>MTVQCKPIPALYTVYVLRSTVRHASLYIGSTPNPPRRLKQHNGLVPGGAARTSRSSLRPWEMVALVSGFPSMVAALKFQWALTNPHLSVHIPSASRLTVATQTKANGRPQRPPRSLASVVANLHLLLRVPSFARWPLRVHFFRRDVFAAWEKWCAAASERLRPSLAVVTDFEGGSEGLAGAVVGGEEGRERGEGAPCWGIHALPLDYEPIKDYVAKGQEIFEFERQGACVVCREEMASGDGLQALCTNQGCDGVGHLSCWSRHFLKGA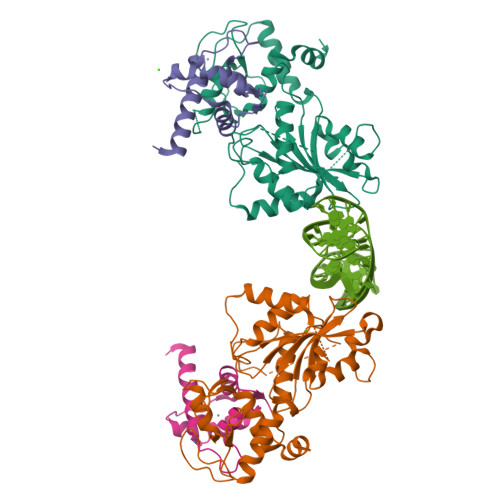EADSILPVQGQCPKCGGEMEWGNMMKELTLRTRGQKEVEKLLKRKRRRATKKTANA[2x];>MEDTETSLVASPTDQQVSLFRYITQAVVTAPRAKDPANPSWHEKMLMYDPIILEDLTAWLNSGQLDRVGYDGEVAPGDVKKWCESKSVCCLWRVSLNGKERKRF[2x]> MSNQGEYPEDNRVGKHEPHDLSLTRRDLIKVSAATAATAVVYPHSTLAASVPAATPAPEIMPLTLKVNGKTEQLEVDTRTTLLDTLRENLHLIGTKKGCDHGQCGACTVLVNGRRLNACLTLAVMHQGAEITTIEGLGSPDNLHPMQAAFIKHDGFQCGYCTSGQICSSVAVLKEIQDGIPSHVTVDLVSAPETTADEIRERMSGNICRCGAYANILAAIEDAAGEIKS;> MKAFTYERVNTPAEAALSAQRVPGAKFIAGGTNLLDLMKLEIETPTHLIDVNGLGLDKIEVTDAGGLRIGALVRNTDLAAHERVRRDYAVLSRALLAGASGQLRNQATTAGNLLQRTRCPYFYDTNQPCNKRLPGSGCAALEGFSRQHAVVGVSEACIATHPSDMAVAMRLLDAVVETITPEGKTRSITLADFYHPPGKTPHIETALLPGELIVAVTLPPPLGGKHIYRKVRDRASYAFALVSVAAIIQPDGSGRVALGGVAHKPWRIEAADAQLSQGAQAVYDTLFASAHPTAENTFKLLLAKRTLASVLAEARAQA;> MKFDKPAGENPIDQLKVVGRPHDRIDGPLKTTGTARYAYEWHEEAPNAAYGYIVGSAIAKGRLTALDTDAAQKAPGVLAVITASNAGVLGKGDKNTARLLGGPTIEHYHQAIALVVAETFEQARAAASLVQAHYRRNKGAYSLADEKQAVNQPPEDTPDKNVGDFDGAFTSAAVKIDATYTTPDQSHMAMEPHASMAVWDGNKLTLWTSNQMIDWCRTDLAKTLKVPVENVRIISPYIGGGFGGKLFLRSDALLAALAARAVKRPVKVMLPRPSIPNNTTHRPATLQHLRIGADQSGKITAISHESWSGNLPGGTPETAVQQSELLYAGANRHTGLRLATLDLPEGNAMRAPGEAPGLMALEIAIDELAEKAGIDPVEFRILNDTQVDPAGPTRCFSRRQLIECLRTGADKFGWKQRNATPGQVRDGEWLVGHGVAAGFHNNLLEKSGARVHLEQNGTVTVETDMTDIGTGSYTILAQTAAEMLGVPLEQVAVHLGDSSFPVSAGSGGQWGANTSTSGVYAACMKLREMIASAVGFDPEQSQFADGKITNGTRSATLHEATAGGRLTAEESIEFGTLSKEYQQSTFAGHFVEVGVHSATGE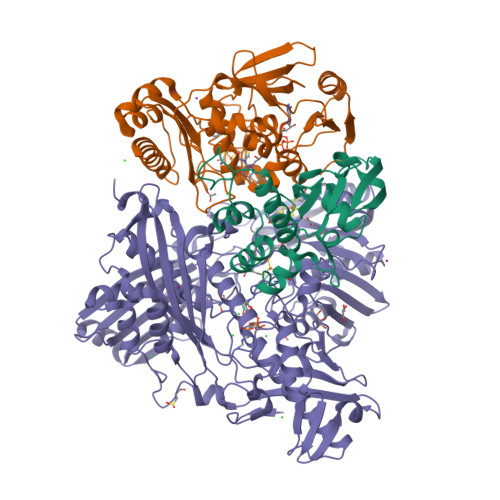VRVRRMLAVCAAGRILNPKTARSQVIGAMTMGMGAALMEELAVDDRLGYFVNHDMAGYEVPVHADIPKQEVIFLDDTDPISSPMKAKGVGELGLCGVSAAIANAVYNATGIRVRDYPITLDKLLDKLPDVV> AQDDSTPDSLFAGLVGEYYGTNSQLNNISDFRALVDSKEADATFEAANISYGRGSSDVAKGTHLQEFLGSDASTLSTDPGDNTDGGIYLQGYVYLEAGTYNFKVTADDGYEITINGNPVATVDNNQSVYTVTHASFTISESGYQAIDMIWWDQGGDYVFQPTLSADGGSTYFVLDSAILSSTGETPYT

MpPA14 (Marinomonas primoryensis PA14 domain) lectin is a domain of a 1.5-MDa adhesin responsible for a symbiotic bacterium-diatom interaction in Antarctica. Bioinformatic analyses indicated the presence of an ∼20-kDa domain near the C terminus of MpIBP that is a member of the PA14 family, which is a carbohydrate-binding lectin module widely distributed across several kingdoms of life. PA14 domains share a β-sandwich fold and the presence of two consecutive aspartate residues in a cis peptide linkage (DcisD). The DcisD motif coordinates a Ca2+ ion that is directly involved in binding polar vicinal hydroxyl groups of various carbohydrates.

Glucose, GlcNAc, and other glucopyranose-containing carbohydrates, including 2-deoxy-glucose, methyl-α-glucose, and two disaccharides (sucrose and trehalose), all bound to the Mp-PA14-Ca1 via their trans vicinal 3,4-diols (ionic bond length, 2.5 Å) in gauche configuration with a dihedral angle of ∼60°. This interaction is further enhanced with the diol being coordinated by the side chain carboxyl and hydroxyl oxygens of the DcisD motif, and main-chain and side chain protein ligands from L11 (Gln156, Gly157, and Asp159).> NTKYN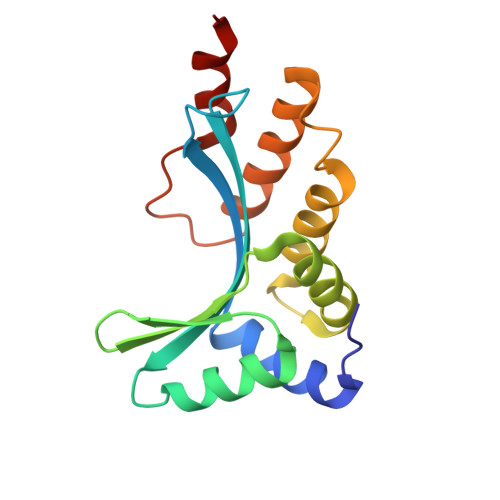KEFLLYLAGFVDSDGSIIAQIKPNQSVKFKHRLQLTFDVTQKTQRRWFLDKLVDEIGVGYVADSGSVSKYRLSEIKPLHNFLTQLQPFLKLKQKQANLVLKIIEQLPSAKESPDKFLEVCTWVDQIAALNDSKTRKTTSETVRAVLDSL In the course of analyzing the structure and interactions of CTLA-4, which is providing important insights into avidity enhancement of regulatory signals at the T-cell surface, we crystallised and solved the structure of an Escherichia coli-expressed monomeric form of the protein (ecCTLA-4), which unexpectedly formed a misfolded dimer and both amyloid and amorphous aggregates under largely physiological conditions. A monomeric form of ecCTLA-4, which comprises a canonical Ig superfamily (IgSF) V-set domain, was engineered by mutating the cysteine at position 122, which forms a disulfide between the C-terminal membrane-proximal linker regions of the protein, to a serine. Immunoglobulin (Ig) light-chain protein deposition diseases arise when Ig domains form pathology-inducing aggregates; these can occur in a variety of organs but most frequently in the kidney. Our work provides new insights into the stability of immunoglobulin folds and the process by which they form disease-inducing amyloid-like deposits.

As expected, this construct was expressed as a monomer, and its crystal structure revealed the characteristic V-set IgSF fold. Although only one molecule of CTLA-4 is present in each crystallographic asymmetric unit, an unexpected swapping of the C-terminal β-strands between adjacent ecCTLA-4 molecules results in the formation of an artificial homodimer (compare the topology diagrams in Fig. 1b and c). The GG′ strands of one domain replace the GG′ strands of a neighbour, and vice versa, forming a compact dimeric unit. A structural comparison with the native, non-strand-swapped crystal structures of B7-complexed CTLA-43 and mammalian-expressed CTLA-4 (maCTLA-4; Yu et al., manuscript in preparation) which forms a quite different disulfide-linked dimer, revealed that cis–trans isomerisation of the prolines at positions 101 and 103 relieves peptide bond strain in ecCTLA-4 seemingly driving the strand swap of the C-terminal β-strands. As well as this reconfiguration, new van der Waals and hydrogenbonding interaction networks between the amino acids forming the (opened) hinging region appear to provide stabilisation energy for the strand-swapped ecCTLA-4 dimer, alongside the formation of the native-like β-strand interactions between the GG′ and F strands. The strand swap seen in our CTLA-4 structure is strikingly similar to that found for CD478 and also that seen for a llama antibody variable heavy chain, which was hypothesised to provide a basis for understanding aggregation by Ig domains. To investigate the possibility that the strand swapping we observe could underpin additional levels of aggregation, we incubated a concentrated solution of monomeric ecCTLA-4 at room temperature for 24 h, whereupon dimeric and larger oligomeric species formed. This indicates that purified monomeric ecCTLA-4 ectodomain can refold to a relatively stable strand-swapped dimer and also produce larger aggregates.

> MKAMHVAQPAVVLASSRGIASFVCEYASPGKATEVRVTVLRQADSQVTEVCAATYMMGNELTFLDDSICTGTSSGNQVNLTIQGLRAMDTGLYICKVELMYPPPYYLGIGNGTQIYVIDPEPSPDSDLVPR>[4x]GPGSMNLSEAPKEIDGHGLLKGKVVLVTAAAGTGIGSTTARRALLEGADVVISDYHERRLGETRDQLADLGLGRVEAVVCDVTSTEAVDALITQTVEKAGRLDVLVNNAGLGGQTPVVDMTDEEWDRVLNVTLTSVMRATRAALRYFRGVDHGGVIVNNASVLGWRAQHSQSHYAAAKAGVMALTRCSAIEAVEFGVRINAVSPSIARHKFLEKTSSSELLDRLASDEA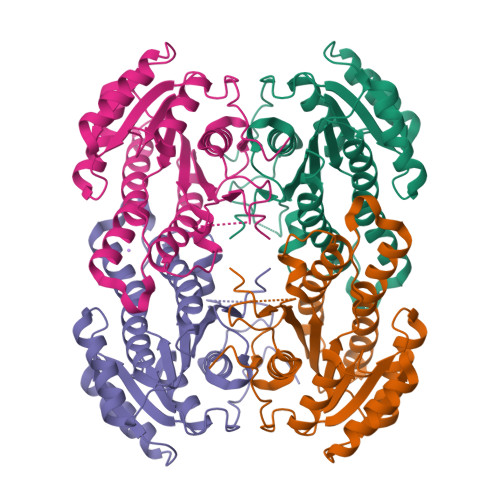FGRAAEPWEVAATIAFLASDYSSYMTGEVVSVSSQRA> KSTQATL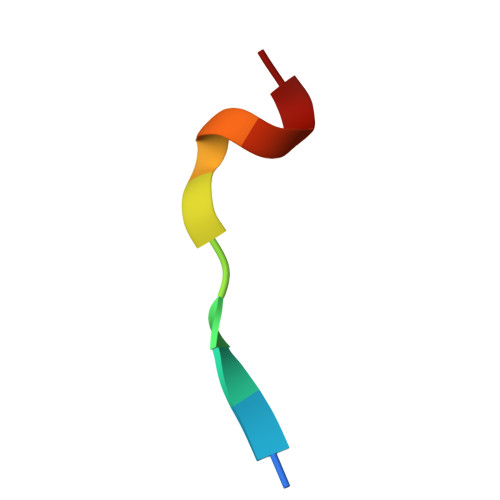ERWF> RRF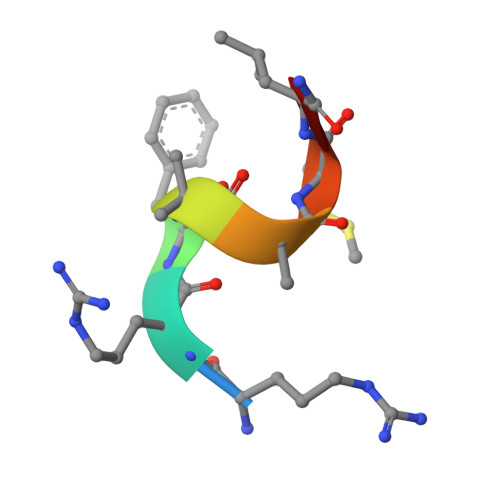AAMLA RBP, via its second and third SH3 domain, is known to bind synaptic ligands such as Ca2+ channels and RIM. Drosophila RBP SH3-II and -III share 49.2% sequence identity and adopt the canonical fold of SH3 domains. We observed the classical poly-proline helix that allows for mainly hydrophobic protein-peptide interaction in all three structures. In summary, we find that the SH3-II and -III interaction surface of RBP serves as a multi-functional platform for differential protein interaction with either other AZ components or the transport adaptor and therefore, motor-cargo linkage.

Finally, in order to get a deeper atomic insight into the structural basis of the binding of RBP towards Aplip1 in comparison to its synaptic ligands, we crystallized the Drosophila RBP SH3-II domain together with both an Aplip1 and a Cac peptide, and RBP SH3-III with a Cac peptide. We detected the same hydrogen pattern between the protein side chains and peptide backbone in the structure of SH3-II with Aplip1 and Cac. The major difference is the side chain orientation of R1687 of Cac that π-stacks with its guanidinium function with Y1372, except for one copy, where it forms a salt-bridge to E1341. A second major difference is induced by the two consecutive proline residues in the Cac peptide. Consequently, the peptide has a more polyproline type II conformation that brings T1692 closer to the protein surface and allows P1693 to deeper point in a hydrophobic pocket of the SH3-II domain. The side chain orientation of Cac R1687 is again different if bound to SH3-II or SH3-III. Completeness of the model given for the six complexes of RBP SH3-II and the bound Cac peptide 1685IGRRLPPTPSKPSTL1699.

>GPLGSPEFRYFVAMFDYDPSTMSPNPDGCDEELPFQEGDTIKVFGDKDADGFYWGELRGRRGYVPHNMVSEVE[10x];>[10x]XIGRRLPPTPSKPSTLX>THTPKLKHLDKLLAHCHRRRYTAKSTIIYAGDRCETLFFIIKGSVTILIEDDDGREMIIGYLNSGDFFGELGLFEKEGSEQERSAWVRAKVECEVAEISYAKFRELSQQDSEILYTLGSQMADRLRKTTRKVGDLAFLDVTGRVART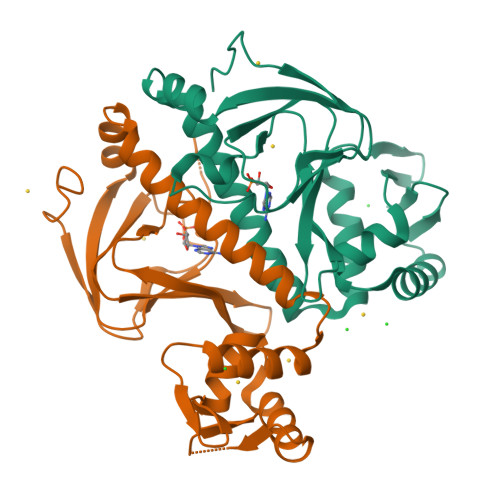LLDLCQQPDAMTHPDGMQIKITRQEIGRIVGCSREMVGRVLKSLEEQGLVHVKGKTMVVFGTR[8x]(2S,3R)-2-[(2S,3R)-1,3-bis(oxidanyl)-1-oxidanylidene-butan-2-yl]-4-[(3S,5S)-5-(dimethylcarbamoyl)pyrrolidin-3-yl]sulfanyl-3-methyl-2,3-dihydro-1H-pyrrole-5-carboxylic 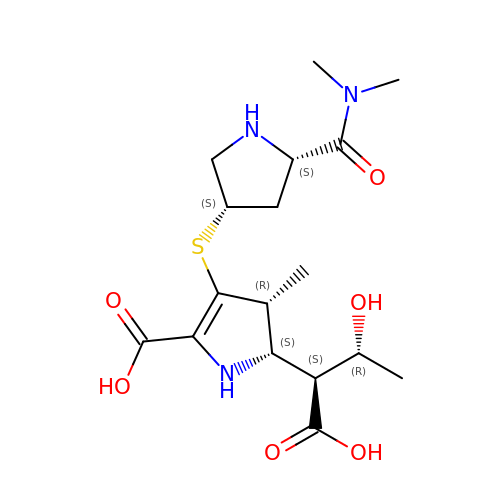acid | C17 H27 N3 O6 S | ILVWWUFTACAPIZ-PQTSNVLCSA-N> GHMGVDTLPPPDPNPPREEFNYTVGFKDLNESLNALEDQDLDALMADLVADISEAEQRTIQAQKESSQNQPELLSKEEEEAKAKADKIKLALEKLKEAKVKKLVVKVHMDDSSTKSLMVDERQLARDVLDNLFEKTHCDCNVDWCLYEIYPELQIERVFEDHENVVEVLSDWTRDTENKVLFLEKEERYAVFKNPQNFYLDNKGKKENKETNEKMNAKNKEYLLEESFCGTSIIVPE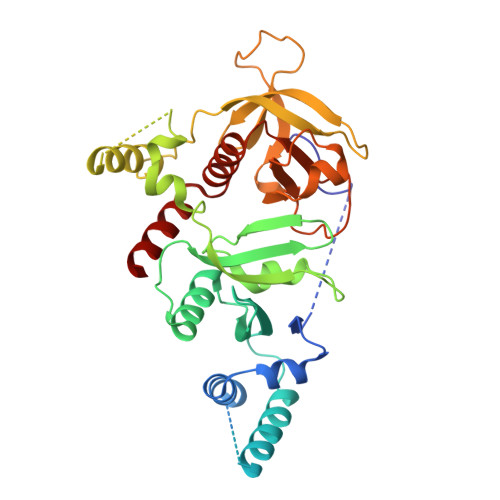LEGALYLKEDGKKSWKRRYFLLRASGIYYVPKGKTKTSRDLACFIQFENVNIYYGIQCKMKYKAPTDHCFVLKHPQIQKESQYIKYLCCDDARTLSQWVMGIRIAKYGKTLYDNYQRAVARA N-BUTYL-BENZENESULFONAMIDE | 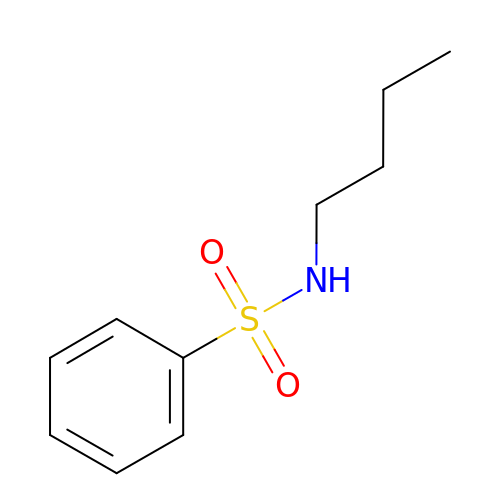C10 H15 N O2 S | IPRJXAGUEGOFGG-UHFFFAOYSA-N> MTRSSAPVSVAVAALLLSAGARPAHAQHLPDLVTQDVLRVCSDPGNMPFSERKGGGFENK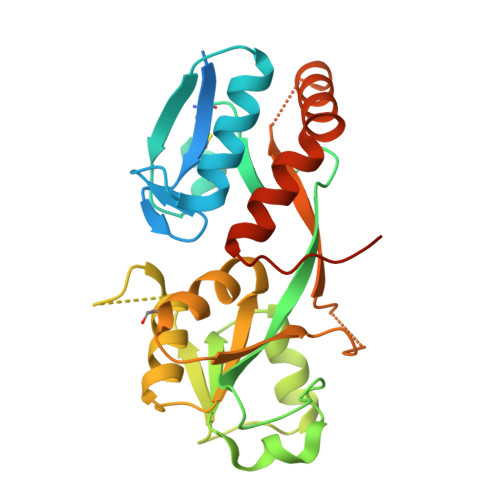IAQIVADELKVKLRYYWLTQGPGFVRNTLGTGLCDLIIGTSGGDIVQATNPYYRSAYVLVARKGELADLKRLDDPRLKDRQIGIIAGTPPSNRLSELKLVGERIHAYAPYAFGAERKHQTVAAEVIADLAEKKIDVAILWGPAAGWLAKQSGVPMDVVPLLHEPGRPPLTFRVSMGVRHNENDWKRSLNTVLRKRKADIEAVLREYEVPLLAEEDTKPLDAADE> INQVRPKLPLLKILHAAGAQGEMFTVKEVMHYLGQYIMVKQLYDAAAQHMVYCGGDLLGELLGRQSFSVKDPSPLYDMLRKNLVT;>EFW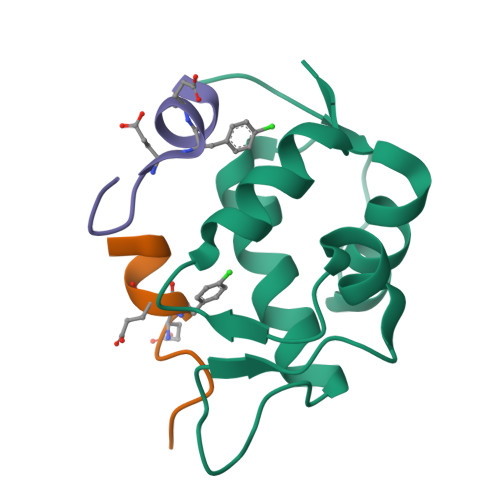YVEXEKLLR[2x]>[2x]AGMQKQVKISGKSKENMSLLKHLKGDVQGKELVIEDSIVNERWKQVLKEKIDIEHDLFNYQKNREISKVPFLPVDRLITNDEVEDILNTLTEVLPTGKFTSGPYLEQFEKVLSTYLHKRYVIATSSGTDAIMIGLLALG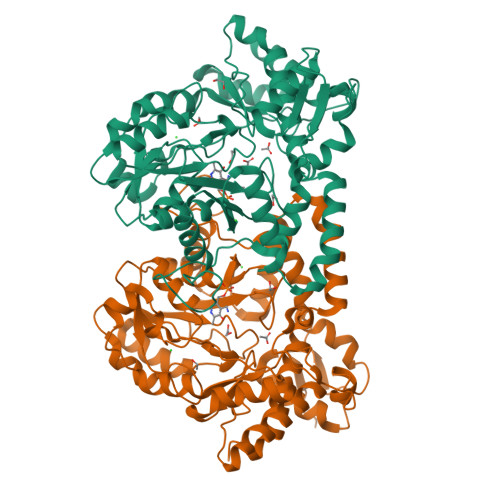LNPGDEVIMPANSFSATENAVLASGGVPIYVDINPQTFCIDPDKIEEAITPYTKFILPVHLYGKHSDMQHIRQIANRYKLKVIEDACQGIGLTDLGKYADITTLSFNPYKNFGVCGKAGAIATDNEELAKKCIQFSYHGFEVNVKNKKVINFGFNSKMDNLQAAIGLERMKYLSLNNFKRLFLADRYITQLAELQNKGYIELPELSEDHVWHLFPIKVRTEDRADIMTKLNEDFGVQTDVYYPILSHMQKTPLVQDKYAGLQLVHTEKAHSQVLHLPLYPSFTLEEQDRVMEGLFHVIKQEIGV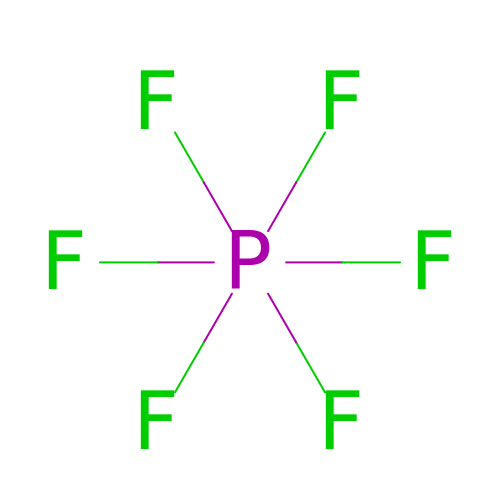Hexafluorophosphate anion | F6 P | WBPJDOUFWQVMRN-UHFFFAOYSA-N> MEAGITGTWYNQLGSTF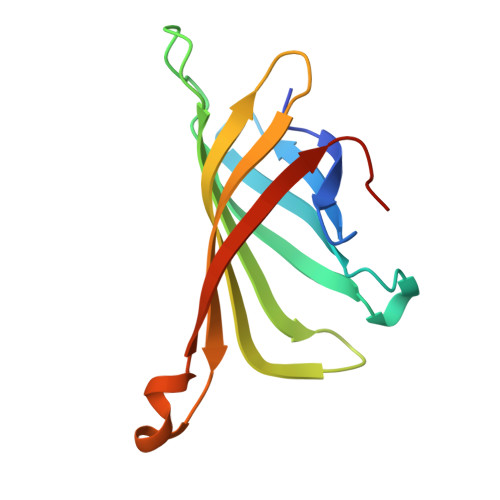IVTAGADGALTGTYIGARGNAESRYVLTGRYDSAPATDGSGTALGWTVAWKNNYRNAHSATTWSGQYVGGAEARINTQWLLTSGTTEANAWKSTLVGHDTFTKVKPSAAS>[4x]MLYYVSILLMAVYAVAVADEDPMTCDKLPKVPVPPLEEFIKSNPLQFAYVLTDTFDCTTRVYVQPARLSPNQAATALDIRGSRIITNDFVGGPNNSAILNNCTTGEKA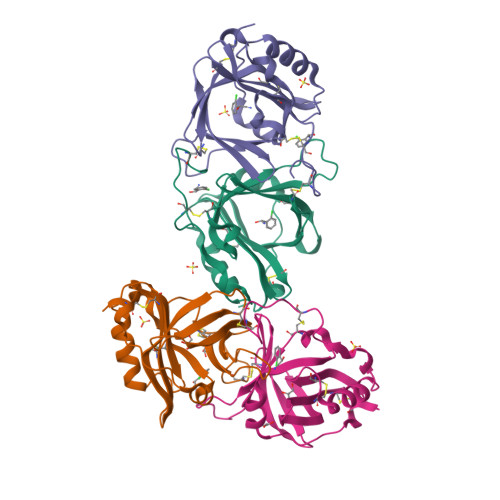TWYFQYTNLNTPNGSSYCAYTCNGEEIAEYKCANNNNGTDPLQKQAVEVAKKVPNGDKIHYALDNCPEHHGCFAFY> GTTLTRQDLNFGQVVADVLCEFLEVAVHLILYVREVYPVGIFQKRKKYNVPVQMSCHPELNQYIQDTLHCVKPLLEKNDVEKVVVVILDKEHRPVEKFVFEITQPPLLSISSDSLLSHVEQLLAAFILKISVCDAVLDHNPPGCTFTVLVHTREAATRNMEKIQVIKDFPWILADEQDVHMHDPRLIPLKTMTSDILKMQLYVEERAHKGSGSGSGSGSGSGSGSGSGSGSKLIG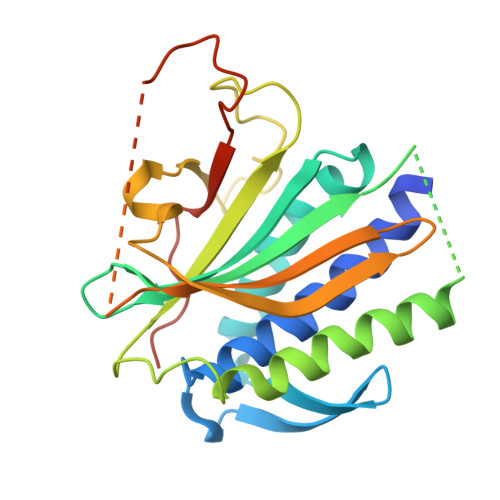DPNLEFVAMPALAPPASREEIMATL> NGDRLYRADSRPPDEIKRSGGLMPRGHNEYFDRGTQMNICLYDHARGTQTGFVRYDDGYVSTSLSLRSAHLAGQSILSGYSTYYIYVIATAPNMFNVNDVLGVYSPHPYEQEVSALGGIPYSQIYGWYRVNFGVIDERLHRNREYRDRYYRNLNIAPAEDGYRLACFPPDHQAWREEPWIHHAPQGCGNSSRTITGDTCNEETQNLSTIYLREYQSKVKRQIFSDYQSEVDIYNRIRDEL;>APQTITELCSEYRNTQIYTINDKILSYTESMAGKREMVI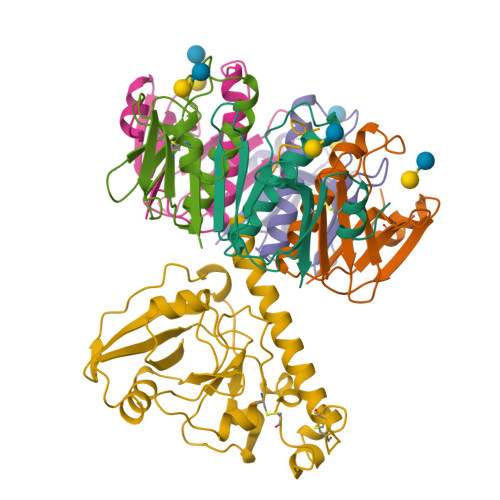ITFKSGETFQVEVPGSQHIDSQKKAIERMKDTLRITYLTETKIDKLCVWNNKTPNSIAAISMKN[5x]In this study we show that IbpS, a protein secreted by D. dadantii, can bind Fe3+ and Cu2+. We demonstrate that exogenously added IbpS reduces the toxicity of H2O2, probably by preventing the Fenton reaction. Our work establishes that members of the Ibp family exhibit the same fold as SBP proteins albeit with significant modifications making of IbpS structure a prototype for this family. The reduced pathogenicities of D. dadantii ibpS and Botrytis cinerea ibp mutants reveal the importance of this conserved protein in the infectious process deployed by necrotrophic microbes probably because of their impaired capacity to detoxify ROS produced during infection.

The crystal structure of the translocated region of D. dadantii IbpS (residues 28–372) was solved at a resolution of 1.7 Å using the single anomalous dispersion method. The asymmetric unit of the crystal contains four chains A, B, C, and D that are nearly identical (rmsd < 0.4 Å). The structure of the IbpS monomer displays a typical SBP fold with two α/β lobes connected by a central hinge region consisting of an extended two-strand β-sheet. The protein displays an additional α-helix at its N terminus and an extended C-terminal tail (residues 352–372) that, to our knowledge, are not observed in the other members of the class II/cluster D family. The C-terminal tail connects the two lobes on the edge of the substrate-binding pocket and appears to stabilize the protein in a conformation similar to a closed state, even in the absence of ligand. Furthermore, the central α-helix in the substrate-binding pocket, which is involved in iron or ligand binding in several class II/cluster D members such as AfuA39 or FutA40 is absent in D. dadantii IbpS structure and replaced by an extended loop. Moreover the ligand-binding pocket is partly occluded by the C-terminal tail and the N-terminal part of α2. We observed two dimers in the crystal formed by A and D’ (symmetry-related of chain D) and B and C’ (symmetry-related of chain C) that were original and not found in other SBP structures to our knowledge. The interface buries 1230 Å2 and is made of electrostatic interactions between α3 from chain A and α15 from chain D’ and vice versa and between the two α15 helices. Several residues involved in the dimerization, including R223 and R337 are strongly conserved, suggesting that dimerization might be a general feature of the Ibp protein family.

>[4x]ATVAPDTRSLDEIYQSALKEGGTVTVYAGGDVQSQQAGFKQAFENRFPGIKLNVIVDYSKYHDARIDNQLATDTLIPDVVQLQTVQDFPRWKKQGVLLNYKPVGWDKVYPEFRDADGAWIGAYVIAFSNLVNTQLLNEKSWPREANDYLRPDLKGNLILAYPNDDDAVLFWYKQIVDKYGWEFVEKLQEQDPVYVRGTNVPGAQITTGKYSATFTSSGALVPAAGSVTRFVLPKTDPFVSWAQRAAIFKQAKHPESAKLYLSWLLDPQTQTQVSRMWSVRTDVAPPAGYKHIWEYSNTRPQAFADFMSDRGAVERFRAQMSLYVGEAKGDPTPGWLGLHPEVPLA> GSMPKPINVRVTTMDAELEFAIQPNTTGKQLFDQVVKTVGLREVWFFGLQYVDSKGYSTWLKLNKKVTQQDVKKENPLQFKFRAKFFPEDVSEELIQEITQRLFFLQVKEAILNDEI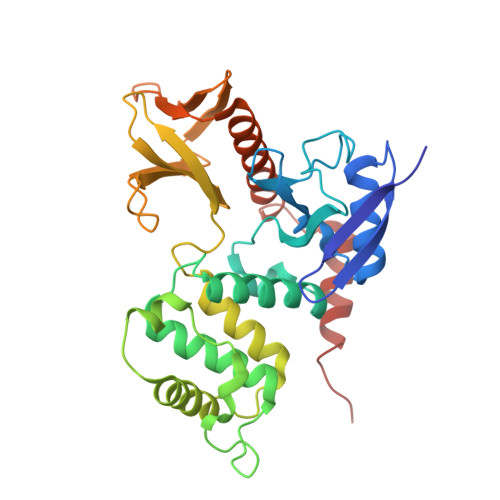YCPPETAVLLASYAVQAKYGDYNKEIHKPGYLANDRLLPQRVLEQHKLTKEQWEERIQNWHEEHRGMLREDSMMEYLKIAQDLEMYGVNYFEIKNKKGTELWLGVDALGLNIYEHDDKLTPKIGFPWSEIRNISFNDKKFVIKPIDKKAPDFVFYAPRLRINKRILALCMGNHELYMRRRKPDTIEVQQMKAQARVDSSGRIVTD> GEVTYRKDIKPIFDVRCAGCHGADAAPEYHAFKAEKEKWLAKGQGMRMDTYSHLIFYTAWPDTGALMRRLDDGKNSKDAKPGNMYRHLGATEEERQRN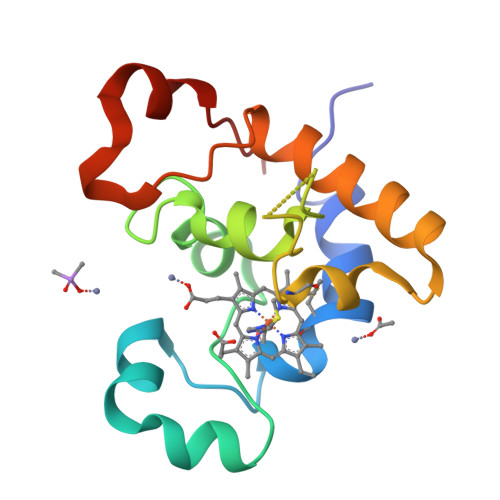LAVFKAWVGVWNLKKWPDITKEELNAITVTY N-cyclohexyl-N~3~-[2-(3,4-dichlorophenyl)ethyl]-N-(2-{[2-(5-hydroxy-3-oxo-3,4-dihydro-2H-1,4-benzoxazin-8-yl)ethyl]amino}ethyl)-beta-alaninamide | C29 H38 Cl2 N4 O4 | 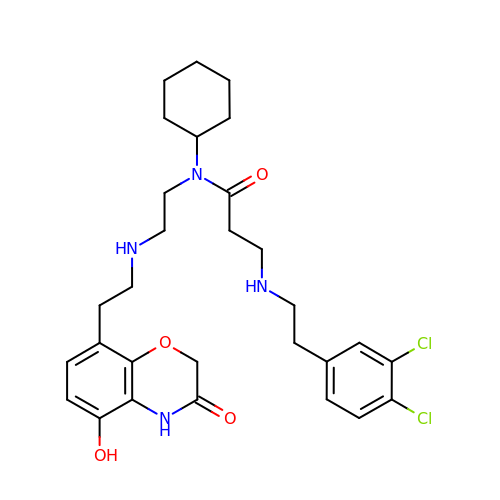LIBVHXXKHSODII-UHFFFAOYSA-N> GSHMASDL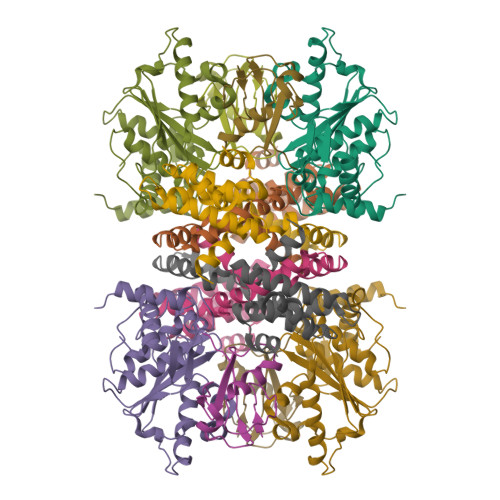LELTEDMEKEISNALGHGPQDEILSSAFKLRITRGDIQTLKNYHWLNDEVINFYMNLLVERNKKQGYPALHVFSTFFYPKLKSGGYQAVKRWTKGVNLFEQEIILVPIHRKVHWSLVVIDLRKKCLKYLDSMGQKGHRICEILLQYLQDESKTKRNSDLNLLEWTHHSMKPHEIPQQLNGSDSGMFTCKYADYISRDKPITFTQHQMPLFRKKMVWEILHQQLL;> MGEGEYIKLKVIGQDSSEIHFKVKMTTHLKKLKESYCQRQGVPMNSLRFLFEGQRIADNHTPKELGMEEEDVIEVYQEQTGG;> SLNTGEPAPVLSSPPPADVSTFLAFPSPEKLLRLGPKSSVLIAQQTDTSDPEKVVSAFLKVSSVFKDEATVRMAVQDAVDALMQKAFNSSSFNSNTFLTRLLVHMGLLKSEDKVKAIANLYGPLMALNHMVQQDYFPKALAPLLLAFVTKPNSALESSSFARHSLLQTLYKV> 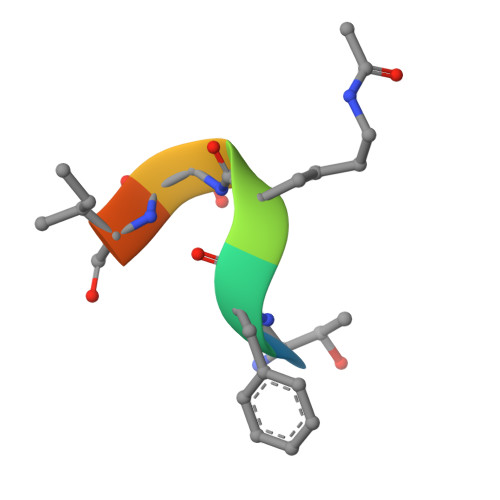TFKSIMK(2S)-2-[2-(4-chlorophenyl)-1H-benzimidazol-1-yl]-N,2-dicyclohexylethanamide | C27 H32 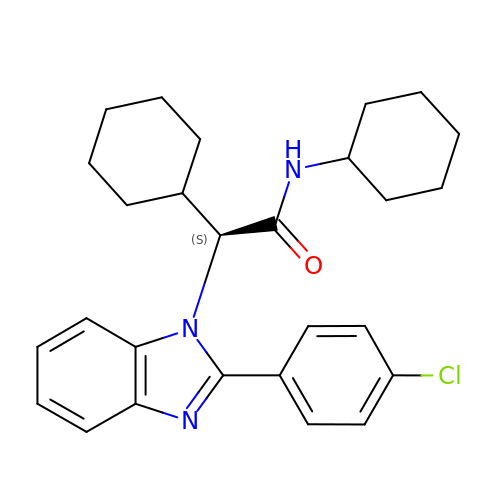Cl N3 O | DZGNRZLPMHOISU-VWLOTQADSA-N> MDETGKELLLVLYDYQEKSPREVTMKKGDIVTLLNSTNKDWWKI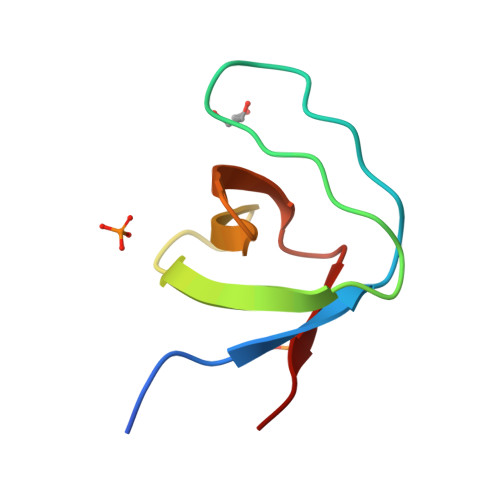EVNDRQGFIPAAYVKKLD> 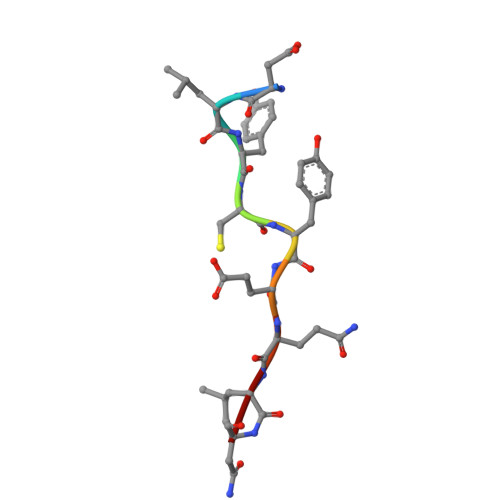DLYCYEQLN> MTCAYRREIHHAHVAIRDWLAGDSRADALDALMARFAEDFSMVTPHGVVLDKTALGELFRSKGGTRPGLRIEIDGESLLASGVDGATLAYREIQSDAAGRSERLSTVVLHRDDEGRLYW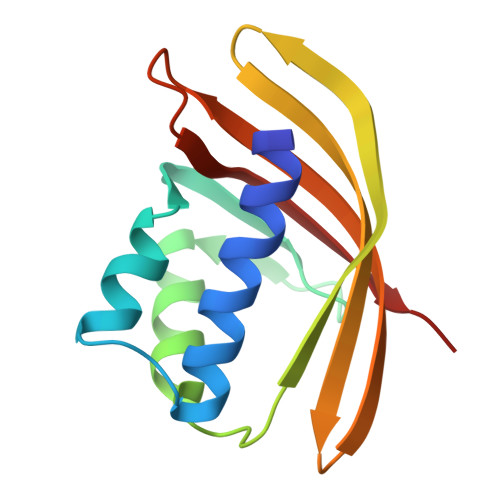RHLQETFCG FzmM and CreE catalyze the triple N-hydroxylation of L-aspartate to nitrosuccinate. The crystal structure of Streptomyces sp. V2 L-aspartate N-hydroxylase outlines a characteristic helical domain wedged between two dinucleotide-binding domains. Together with NADPH and FAD, a cluster of conserved arginine residues forms the catalytic core at the domain interface. The Lineweaver-Burk plot of the initial rates revealed a pattern of lines intercepting on the horizontal axis, suggestive of a ternary complex mechanism. Thus, Streptomyces sp. V2 L-aspartate N-hydroxylase operates as a typical class B flavoenzyme monooxygenase: it is a single-component enzyme that binds simultaneously FAD and NADPH and retains the pyridine nucleotide coenzyme throughout the catalytic process.

Nonetheless, we noticed that the crystals could stand prolonged soakings in solutions comprising sodium tartrate, PEG4000, 15 mM L-aspartate, and 5 mM NADPH with no ammonium sulfate being present. We further observed bleaching of the crystals indicating that the enzyme was reduced by NADPH. This procedure thereby allowed us to solve the structure of the reduced enzyme in complex with NADP(H) and L-aspartate at 2.1 Å resolution. The electron density unambiguously showed the presence of a molecule of L-aspartate with the side chain carboxylate overlapping the position occupied by a sulfate ion. The ligand is engaged by several interactions mainly with the arginine cluster (Arg13, Arg276, Arg416, Arg577, and Asn413). The critical observation is that this position of L-aspartate cannot be conducive to the oxygenation of its amino group which remains too far away (∼10 Å) from the flavin N5-C4a locus. Therefore, we shall refer to this site as an “entry chamber”. For oxygenation to occur, the substrate should bind more deeply, inside the “catalytic” center wedged between the isoalloxazine and the nicotinamide-ribose moiety of NADP(H). We could not detect any bound L-aspartate in this site even after prolonged soaking. In the L-aspartate structure, Asn62 is flipped “outwards”, vacating the space in front of the flavin.

>[2x]MPLSVAVVGAGPRGTSVLERLCASAPELLAPGVRLTVHVVDPAPPGPGRVWRTAQSEDLLMNTVASQVTLFTDESVNCSGPILAGPSLHEWADGAIGPDDYPTRALYGRYLEWVFARTLRHAPPSVRVETHRARAVRLDDAADGRQHLALDNGRTLTGLSAVVLAQGHLPVRPSAAVLRDTEHADRHALRHIPPANPADVDLTVISPGEPVLLRGLGLNFFDHMALLTTGRGGTYVREDGVLRYVPSGREPRVYAGSRRGLPYQARGDNAKGPYGRHLPEVLTPEAVSAFRKRADSGEAPDFLRDIWPLVAKEVETVYYTALVRHPDFAPRYLSLPYGDPQEAELLAEFGVDADARWDWERVSRPYAQREFAHRGEWRQWLLGYLRADAAEALRGNVDGPLKAALDVLRDLRNELRLVVDHRGLRGDSRRDHLDRWYTPLNAFLSIGPPRRRIEELTALLEAGVVEVLGPRLEVTREDGAWLARSPDVPGSAVRVTTLIEARLPEPDLGQTADALLAHLRETGQCRAHVVDGYTTGGIDVSARPYHLVDREGVAHPRRFAFGVPTEGVHWVTAAGARPGVDSVTLSDADAVARAVLRVAGQ> GAMGSMSKSLKKLVEESREKNQPEVDMSDRGISNMLDVNGLFTLSHITQLVLSHNKLTMVPPNIAELKNLEVLNFFNNQIEELPT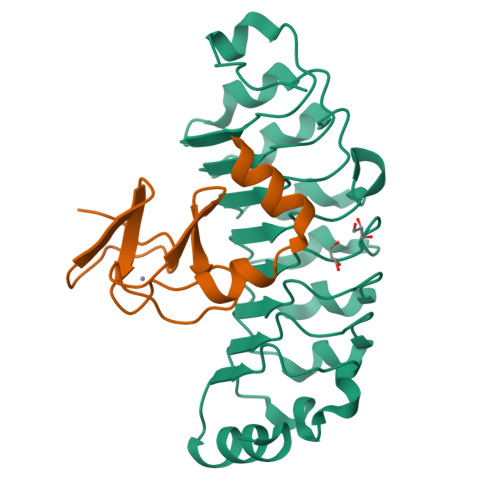QISSLQKLKHLNLGMNRLNTLPRGFGSLPALEVLDLTYNNLSENSLPGNFFYLTTLRALYLSDNDFEILPPDIGKLTKLQILSLRDNDLISLPKEIGELTQLKELHIQGNRLTVLPPELGNLDLTGQKQVFKAEN;> GPGSGDVCFHCNRVIEGDVVSALNKAWCVNCFACSTCNTKLTLKNKFVEFDMKPVCKKCYEKFPLELKKRLKKLAETLGRK> MNENYYISPSLDTLSSYSLLQLRKVPHLVVGHKSYGKIEFLEPVDLAGIPLTSLGGVIITFEPKTCIIYANLPNRPKRGEG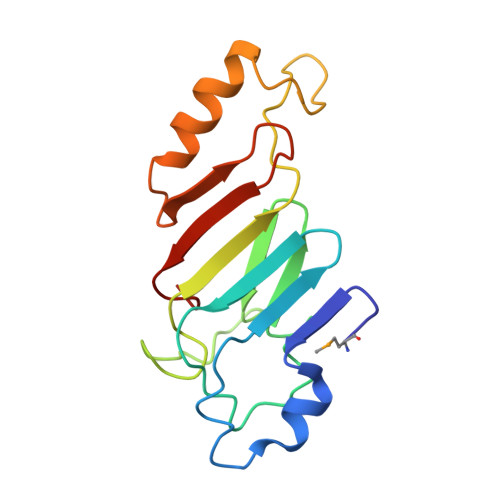INVRARITCFNCYPVDKSTRKPIKDPNHQLVKRHIERLKKNPNSKFESYDADSGTYVFIVNHAAEQT>MK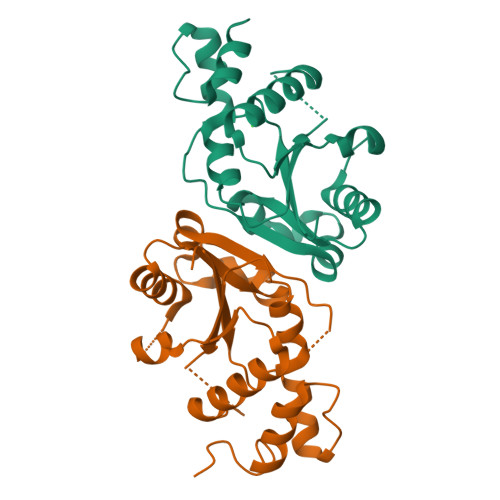KIAIFGSAFNPPSLGHKSVIESLSHFDLVLLEPSIAHAWGKNMLDYPIRCKLVDAFIKDMGLSNVQRSDLEQALYQPGQSVTTYALLEKIQEIYPTADITFVIGPDNFFKFAKFYKAEEITERWTVMACPEKVKIRSTDIRNALIEGKDISTYTTPTVSELLLNEGLYRETLSGK[2x]>MPHFTVTKVEDPEEGAAASISQEPSLADIKARIQDSDEPDLSQNDITGEHSQLLDDGHKKARNAYLNNSNYEEGDEYFDKNLALFEEEMDTRPKVSSLLNRMANYTNLTQGAKEHEEAENITEGKKKPTKTPQMGTFMGVYLPCLQNIFGVILFLRLTWVVGTAGVLQAFAIVLICCCCTMLTAISMSAIATNGVVPAGGSYFMISRALGPEFGGAVGLCFYLGTTFAAAMYILGAIEIFLVYIVPRAAIFHSDDALKESAAMLNNMRVYGTAFLVLMVLVVFIGVRYVNKFASLFLACVIVSILAIYAGAIKSSFAPPHFPVCMLGNRTLSSRHIDVCSKTKEINNMTVPSKLWGFFCNSSQFFNATCDEYFVHNNVTSIQGIPGLASGIITENLWSNYLPKGEIIEKPSAKSSDVLGSLNHEYVLVDITTSFTLLVGIFFPSVTGIMAGSNRSGDLKDAQKSIPIGTILAILTTSFVYLSNVVLFGACIEGVVLRDKFGDAVKGNLVVGTLSWPSPWVIVIGSFFSTCGAGLQSLTGAPRLLQAIAKDNIIPFLRVFGHSKANGEPTWALLLTAAIAELGILIASLDLVAPILSMFFLMCYLFVNLACALQTLLRTPNWRPRFRYYHWALSFMGMSICLALMFISSWYYAIVAMVIAGMIYKYIEYQGAEKEWGDGIRGLSLSAARFALLRLEEGPPHTKNWRPQLLVLLKLDEDLHVKHPRLLTFASQLKAGKGLTIVGSVIVGNFLENYGEALAAEQTIKHLMEAEKVKGFCQLVVAAKLREGISHLIQSCGLGGMKHNTVVMGWPNGWRQSEDARAWKTFIGTVRVTTAAHLALLVAKNISFFPSNVEQFSEGNIDVWWIVHDGGMLMLLPFLLKQHKVWRKCSIRIFTVAQLEDNSIQMKKDLATFLYHLRIEAEVEVVEMHDSDISAYTYERDLMMEQRSQ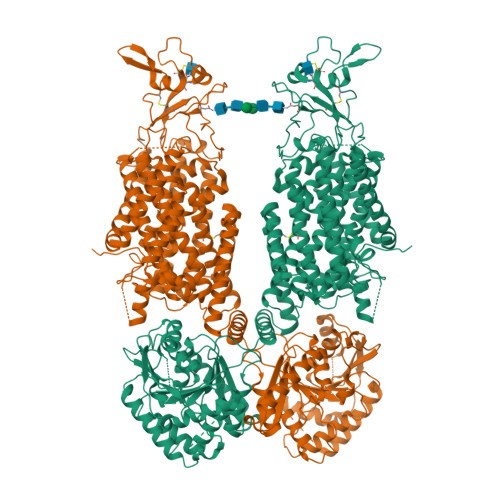MLRHMRLSKTERDREAQLVKDRNSMLRLTSIGSDEDEETETYQEKVHMDWTKDKYMASRGQKAKSMEGFQDLLNMRPDQSNVRRMHTAVKLNEVIVNKSHEAKLVLLNMPGPPRNPEGDENYMEFLEVLTEGLERVLLVRGGGSEVITIYSA[2x]>[4x]MTADKLVFFVNGRKVVEKNADPETTLLAYLRRKLGLSGTKLGCGEGGCGACTVMLSKYDRLQNKIVHFSANACLAPICSLHHVAVTTVEGIGSTKTRLHPVQERIAKSHGSQCGFCTPGIVMSMYTLLRNQPEPTMEEIENAFQGNLCRCTGYRPILQGFRTFARDGGCCGGDGNNPNCCMNQKKDHSVSLSPSLFKPEEFTPLDPTQEPIFPPELLRLKDTPRKQLRFEGERVTWIQASTLKELLDLKAQHPD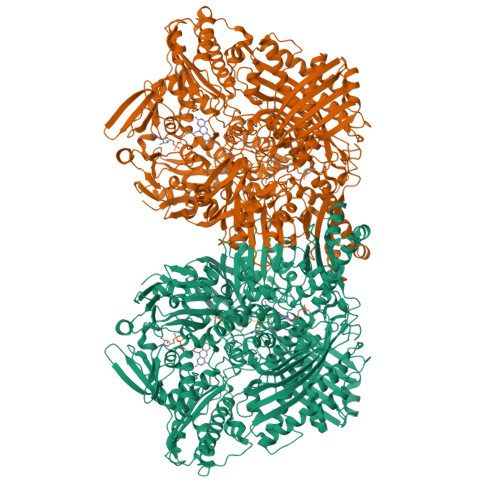AKLVVGNTEIGIEMKFKNMLFPMIVCPAWIPELNSVEHGPDGISFGAACPLSIVEKTLVDAVAKLPAQKTEVFRGVLEQLRWFAGKQVKSVASVGGNIITASPISDLNPVFMASGAKLTLVSRGTRRTVQMDHTFFPGYRKTLLSPEEILLSIEIPYSREGEYFSAFKQASRREDDIAKVTSGMRVLFKPGTTEVQELALCYGGMANRTISALKTTQRQLSKLWKEELLQDVCAGLAEELHLPPDAPGGMVDFRCTLTLSFFFKFYLTVLQKLGQENLEDKCGKLDPTFASATLLFQKDPPADVQLFQEVPKGQSEEDMVGRPLPHLAADMQASGEAVYCDDIPRYENELSLRLVTSTRAHAKIKSIDTSEAKKVPGFVCFISADDVPGSNITGICNDETVFAKDKVTCVGHIIGAVVADTPEHTQRAAQGVKITYEELPAIITIEDAIKNNSFYGPELKIEKGDLKKGFSEADNVVSGEIYIGGQEHFYLETHCTIAVPKGEAGEMELFVSTQNTMKTQSFVAKMLGVPANRIVVRVKRMGGGFGGKVTRSTVVSTAVALAAYKTGRPVRCMLDRDEDMLITGGRHPFLARYKVGFMKTGTVVALEVDHFSNVGNTQDLSQSIMERALFHMDNCYKIPNIRGTGRLCKTNLPSNTAFRGFGGPQGMLIAECWMSEVAVTCGMPAEEVRRKNLYKEGDLTHFNQKLEGFTLPRCWEECLASSQYHARKSEVDKFNKENCWKKRGLCIIPTKFGISFTVPFLNQAGALLHVYTDGSVLLTHGGTEMGQGLHTKMVQVASRALKIPTSKIYISETSTNTVPNTSPTAASVSADLNGQAVYAACQTILKRLEPYKKKNPSGSWEDWVTAAYMDTVSLSATGFYRTPNLGYSFETNSGNPFHYFSYGVACSEVEIDCLTGDHKNLRTDIVMDVGSSLNPAIDIGQVEGAFVQGLGLFTLEELHYSPEGSLHTRGPSTYKIPAFGSIPIEFRVSLLRDCPNKKAIYASKAVGEPPLFLAASIFFAIKDAIRAARAQHTGNNVKELFRLDSPATPEKIRNACVDKFTTLCVTGVPENCKPWSVRV>MGRIKNKQFAVIGLGAFGGSICKELHRMGHEVLAVDINEEKVNAYASYATHAVIANATEENELLSLGIRNFEYVIVAIGANIQASTLTTLLLKELDIPNIWVKAQNYYHHKVLEKIGADRIIHPEKDM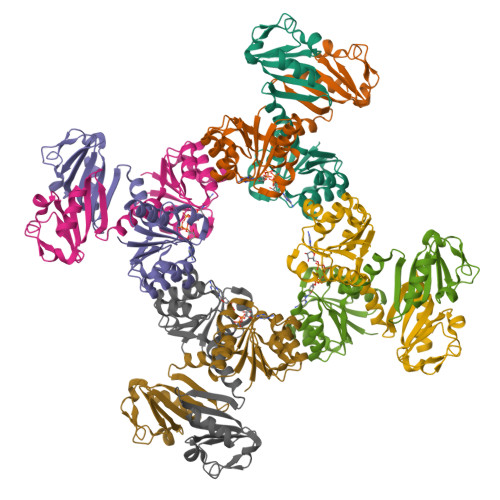GVKIAQSLSDENVLNYIDLSDEYSIVELLATRKLDSKSIIDLNVRAKYGCTILAIKHHGDICLSPAPEDIIREQDCLVIMGHKKDIKRFENEGM[16x]> ELQKSIGHKPEPTDEEWELIKTVTEAHVATNAQGSHWKQKRKFLPEDIGQAPIVNAPEGGKVDLEAFSHFTKIITPAITRVVDFAKKLPMFCELPCEDQIILLKGCCMEIMSLRAAVRYDPESETLTLNGEMAVTRGQLKNGGLGVVSDAIFDLGMSLSSFNLDDTEVALLQAVLLMSSDRPGLACVERIEKYQDSFLLAFEHYINYRKHHVTHFWPKLLMKVTDLRMIGACHASR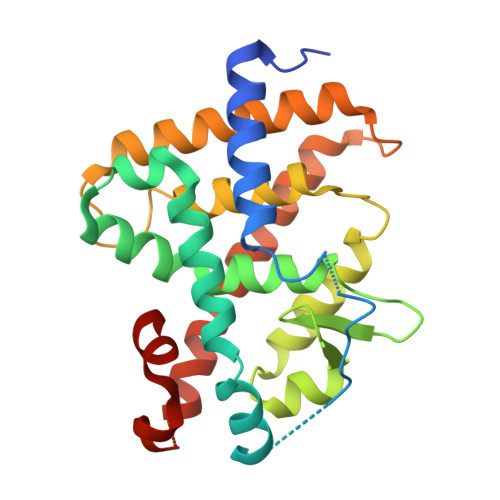FLHMKVECPTELFPPLFLEVFED>MPFRRTLLAASLALLITGQAPLYAAPPLSMDNGTNALTVQNSNAWVEVSASALQHNIRTLQAELAGKSRLCAVLKADAYGHGIGLVMPSIIAQGVPCVAVASNEEARVVRASGFTGQLVRVRLASLSELEDALQYDMEELVGSAEFARQVDAIAARHGKTLRIHMALNSSGMSRNGVEMATWSGRGEALQITDQKHLKLVALMTHFAVEDKDDVRKGLAAFNEQTDWLIKHAKLDRSKLTLHAANSFATLEVPEARLDMVRTGGALFGDTVPARTEYQRAMQFKSHVAAVHSYPAGNTVGYDRTFTLARDSRLANITVGYSDGYRRVFTNKGHVLINGHRIPVVG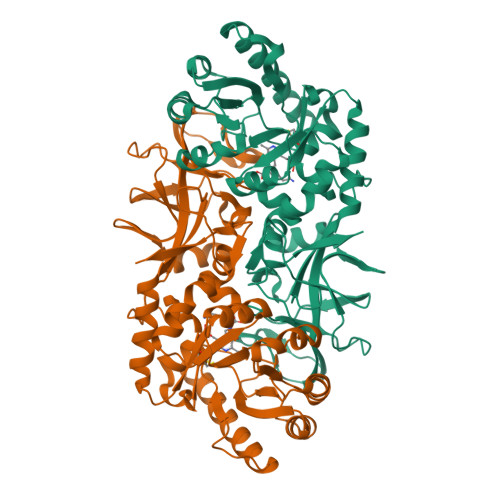KVSMNTLMVDVTDFPDVKGGNEVVLFGKQAGGEITQAEMEEINGALLADLYTVWGSSNPKILVD[2x]>MTSVRENILFGMGNPLLDISAVVDKDFLDKYSLKPNDQILAEDKHKELFDELVKKFKVEYHAGGSTQNSIKVAQWMIQQPHKAATFFGCIGIDKFGEILKRKAAEAHVDAHYYEQNEQP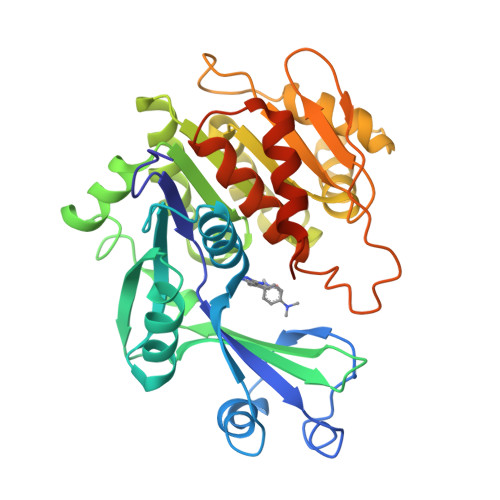TGTCAACITGDNRSLIANLAAANCYKKEKHLDLEKNWMLVEKARVCYIAGFFLTVSPESVLKVAHHASENNRIFTLNLSAPFISQFYKESLMKVMPYVDILFGNETEAATFAREQGFETKDIKEIAKKTQALPKMNSKRQRIVIFTQGRDDTIMATESEVTAFAVLDQDQKEIIDTNGAGDAFVGGFLSQLVSDKPLTECIRAGHYAASIIIRRTGCTFPEKPDFH[2x]> SMTCPFYKKIPGTGFTVDAFQYGVVEGCTAYFLTHFHSDHYAGLSKHFTFPVYCSEITGNLLKNKLHVQEQYIHPLPLDTECIVNGVKVVLLDANHCPGAVMILFYLPNGTVI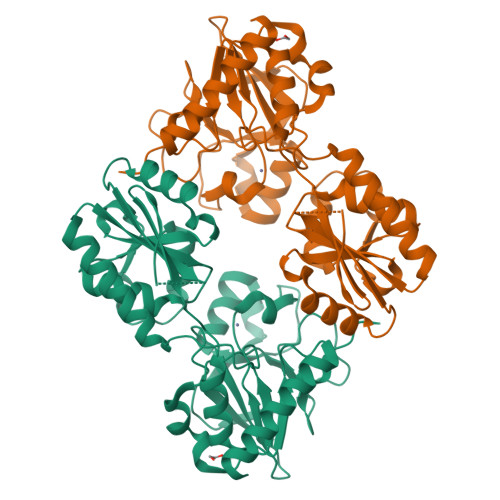LHTGDFRADPSMERSLLADQKVHMLYLDTTYCSPEYTFPSQQEVIRFAINTAFEAVTLNPHALVVCGTYSIGKEKVFLAIADVLGSKVGMSQEKYKTLQCLNIPEINSLITTDMCSSLVHLLPMMQINFKGLQSHLKKCGGKYNQILAFRPTGWTHSNKFTRIADVIPQTKGNISIYGIPYSEHSSYLEMKRFVQWLKPQKIIPTVNVGTWKSRSTMEKYFREWKLEAGY Here we describe a systematic approach to generating modular and rigid repeat protein oligomers with coincident C2 to C8 and superhelical symmetry axes that can be readily extended by repeat propagation. Repeat proteins are composed of an asymmetric structural motif that is concatenated several times in tandem within a single protein chain. From these building blocks, we demonstrate that a wide range of unbounded fibres can be systematically designed by introducing hydrophilic surface patches that force staggering of the monomers; the geometry of such fibres can be precisely tuned by varying the number of repeat units in the monomer and the placement of the hydrophilic patches. All multiplexes follow the naming convention CsHRN_Rr where s is the cyclic symmetry, HR stands for helical repeat, R is the number of repeats in a single chain and N is an index to differentiate between multiplexes of the same symmetry.

We also expressed a C2 dimer directly as an eight-repeat duplex (C2HR4_8r), and the structure by X-ray crystallography to be close to the design model (r.m.s.d. compared with design model = 3.78 Å). The twist of the crystal structure is approximately 22.5° per repeat or 16 repeats per turn, and hence by propagating this structure from 9 to 17 repeats, the angle between the N and C terminal repeats can be modulated from 180° to 360°.

>MGDSEVDKAVSLVEELAQKSGSENAREAAKEIRKRGDSEVALAVALVLSLANKSGSRNAIEAAAEIAKRGDSEVALAVALVLSLANKSGSRNAIEAAAEIAKRGDSEVALAVALVLSLANKSGSRNAIEAAAEIAKRGDSEVALAVALVLSLANKSGSRNAIEAAAEIAKRGDSEVALAVALVLSLANKSGSRNAIEAAAEIAKRGDSEVALAVALVLSLANKSGSRNAIEAAAEIAKRGDSEVALKVALELSQANKNGSRDEIEKAAENAKRGDGWLEHHHHHH[2x]>GMALQLSREQGITARGSAEIVAEFFSFGINSILYQRGIYPSETFTRVQKYGLTLLVTTDLELIKYLNNVVEQLKDWLYKSSVQKLVVVISNIESGEVLERWQFDIESDKTAKDDSAPREKSQKAIQDEIRSVIRQITATVTFLPLLEVSCSFDLLIYTDKDLVVPEKWEESGPQFITNSEEVRLR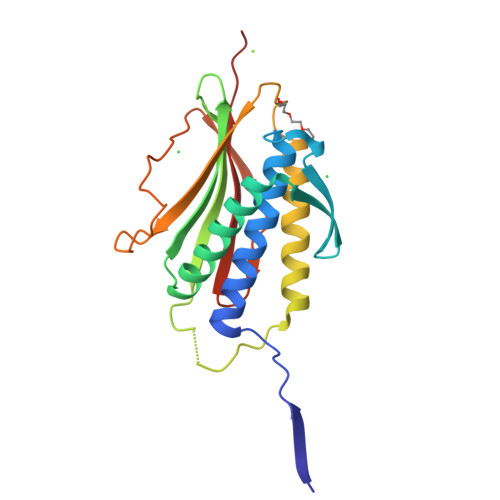SFTTTIHKVNSMVAYKIPVND[12x]> ICIC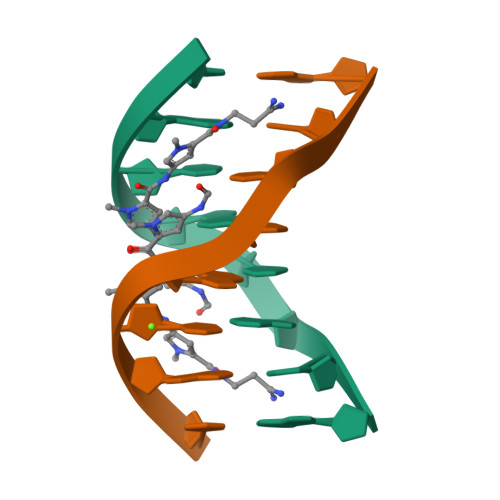ICIC>GHMEGLAGYVYKAASEGKVLTLAALLLNRSESDIRYLLGYVSQQGGQRSTPLIIAARNGHAKVVRLLLEHYRVQTQQTGTVRFDGYVIDGATALWCAAGAGHFEVVKLLVSHGANVNHTTVTNSTPLRAACFDGRLDIVKYLVENNANISIANKYDNTCLMIAAYKGHTDVVRYLLEQRADPNAKAHCGATALHFAAEAGHIDIVKELIKWRAAIVVNGHGMTPLKVAAESCKADVVELLLSHADCDRRSRIEALELLGASFANDRENYDIIKTYHYLYLAMLERFQDGDNILEKEVLPPIHAYGNRTECRNPQELESIRQDRDALHMEGLIVRERILGGGGSGGG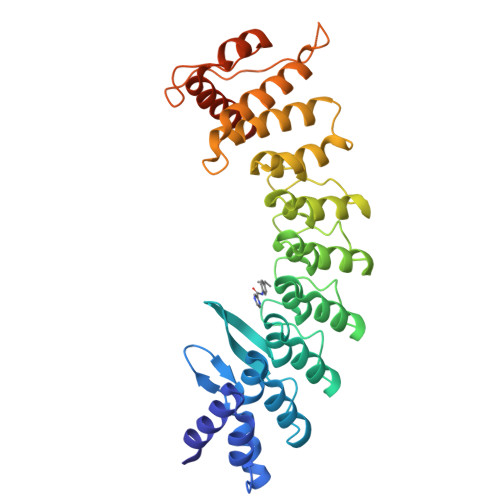SKKRLLLGLDR[2x]>SSGSANFAGVEYPLLPLDQHTPLLFQWFERNPSRFGENQIPIINTQQNPYLNNIINAAIIEKERTIGVLVDGNFSAGQKKALAKLEKQYENIKVIYNSDLDYSMYDKKLSDIYLENIAKIEAQPANVRDEYLLGEIKKSLNEVLKNNPEESLVSSHDKRLGHVRFDFYRNLFLLKGSNAFLEAGKHGCHHLQPGGGCIYLDADMLLTGKLGTLYLPDGIAVHVSRKGNSMSLQNGIIAVNRSEHPALKKGLEIMHSKPYGDPYIDGVCGGLRHYFNCSIRHNYEEFCNFIEFKHEHIFMDTSSLTISSWR[2x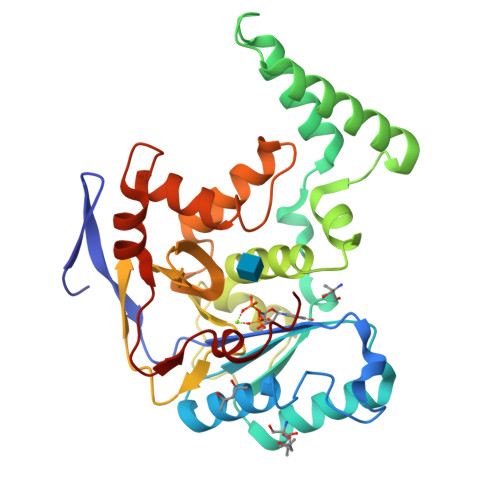]>[2x]PSMKERQVCWGARDEYWKCL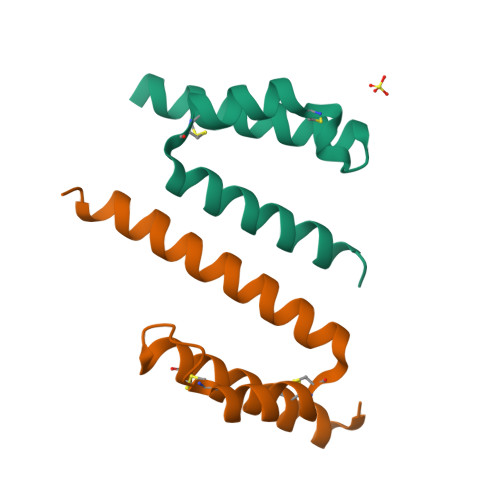DENLEDASQCKKLRSSFESSCPQQWIKYFDKRRDYLKFKEKFEAGQFEPS>CPTHADSLNNLANIKREQGNIEEAVRLYRKALEVFPEFAAAHSNLASVLQQQGKLQEALMHYKEAIRISPTFADAYSNMGNTLKEMQDVQGALQCYTRAIQINPAFADAHSNLASIHKDSGNIPEAIASYRTALKLKPDFPDAYCNLAHCLQIVCDWTDYDERMKKLVSIVADQLEKNRLPSVHPHHSMLYPLSHGFRKAIAERHGNLCLDKINVLHKPP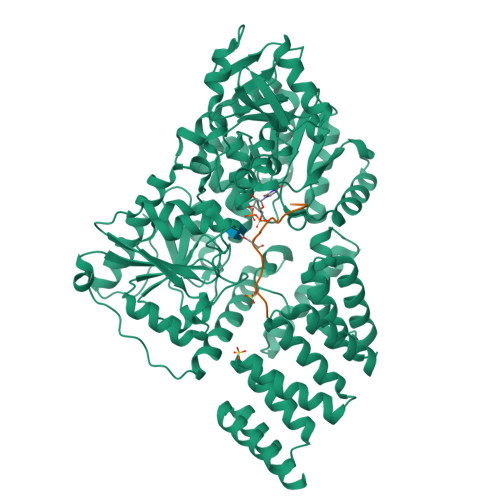YEHPKDLKLSDGRLRVGYVSSNFGNHPTSHLMQSIPGMHNPDKFEVFCYALSPDDGTNFRVKVMAEANHFIDLSQIPCNGKAADRIHQDGIHILVNMNGYTKGARNELFALRPAPIQAMWLGYPGTSGALFMDYIITDQETSPAEVAEQYSEKLAYMPHTFFIGDHANMFPHLKKKAVIDFKSNGHIYDNRIVLNGIDLKAFLDSLPDVKIVKMKCPDGGDNADSSNTALNMPVIPMNTIAEAVIEMINRGQIQITINGFSISNGLATTQINNKAATGEEVPRTIIVTTRSQYGLPEDAIVYCNFNQLYKIDPSTLQMWANILKRVPNSVLWLLRFPAVGEPNIQQYAQNMGLPQNRIIFSPVAPKEEHVRRGQLADVCLDTPLCNGHTTGMDVLWAGTPMVTMPGETLASRVAASQLTCLGCLELIAKNRQEYEDIAVKLGTDLEYLKKVRGKVWKQRISSPLFNTKQYTMELERLYLQMWEHYAAGNKPDHMIKPVE[2x];>[2x]YPGGSTPVSSANMM>MAQRGIREYDAKNLLARYLPEYLDDFSYKGNLALVGPETDIEGLEAENPWLKTTRLVVKPDQLFGKRGKLGLVLLDADWEEAKEYLNEKMGLEVTIGGITGRLSYFLIEPFTPHKEEYYVAISSDYEGDNIFFSMDGGVGVEENWEKVISIHVDSLEGIDALDVGSKLPAELGDKRALVEEFITALWRFYSDTGFAYVEINPFTFSGRGIVPLDMVAKLDDAEEYWQKKRWSELAFPEPFGRTPSKEELFIKEIDSKTGASLKLTILNPEGRVWTMVAGGGASVIYADTICDLGHADEMANYGEYSGDPNTEETYHYTCTILDLMTRSKNPNGKVLLIGGAIANFTDVAKTFKGVVMALEEYQQKLQEADIEIYVRRGGPNYEQGLKLMRDLGKRLGVPIQVHGPETHMTRIVPLALEENQ[2x];>MSRKDYVLFDINTKAFVYGYQTNAIQRMLDFDYVCKRSSPSISAIINPSRAGIHKAFWGTKEIILPMYKTIPLAALAYPEADVMVNFASHRSAFET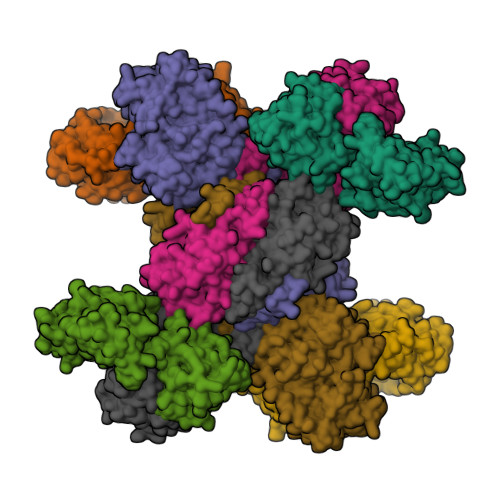TMEALKEDTIRIVAVIAEGVPERQSRVMAATARKLDKIVIGPATVGGMTAGAFRIGNTAGTIENIIASKLYRPGCVGFVSKSGGMLNEAFNIISRNSDGIYEGVAIGGDRYPGSNMLDHILRYERNPAIKMIACLGELGGEDEYMIIQALKEKKITKPLVAWVTGTCSPYLPASVQFGHAGAKANTEKETAQAKNDAFRQAGAYVPRSFDDYGEMVRQVYDMLLTRGIVQKFDEPEVPRIPTDYSKALATGDIRKPTTFICTISDDSGEELLYAGKKLSDVLDRKMGIGGVIGLLWFKKELPEYAAHFIELVIQIVADHGPAVSGAHNAIVASCAGKDLISSLCSGLLTIGPRFGGAIDDAAREFKRAQETGLAPEQFVGEMKKKGINIPGIGHKIKSVKNPDKRVQLLISYARANFPSTELLNYALQVEELTTAKKGNLILNVDGCIGILFIDLMSSCGAFSKEEIDEVVRLGYLNGLFALGRSIGLIGHILDQKRLGSRLYRHPAEDIAYMMPSEEEIQCKRDRGGSHHHHHH[2x]>[2x]MSLTVVLIVDDHHLIRAGAKNLLEGAFSGMR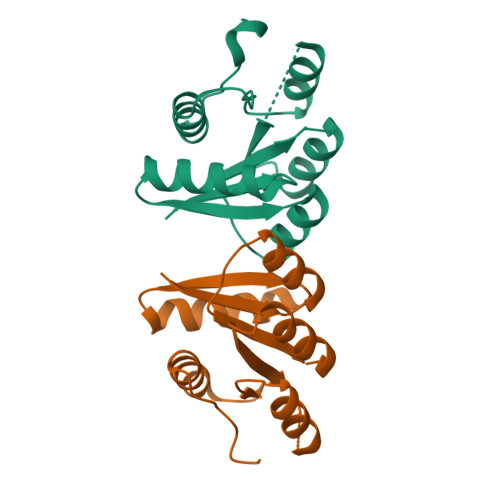VEGAETVSDALAFLEADNTVDLILLDVNLPDAEAIDGLVRLKRFDPSNAVALISGETDHELIRAALEAGADGFIPKSADPQVLIHAVSLILEGEIFLPRSYLQGGRMAEVATPLDEGHHHHHH>[2x]EEDELYRQSLEIISRYLREQATGAKDTKPMGRSGATSRKALETLRRVGDGVQRNHET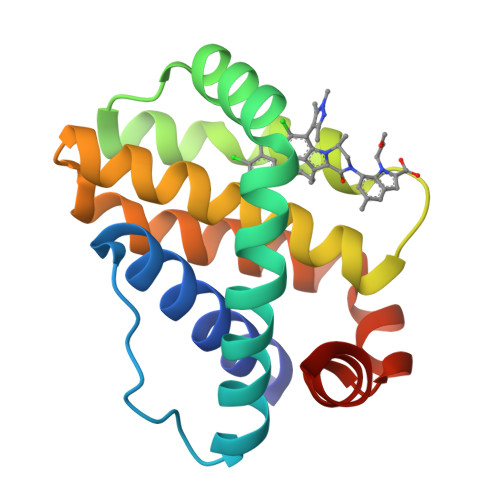AFQGMLRKLDIKNEDDVKSLSRVMIHVFSDGVTNWGRIVTLISFGAFVAKHLKTINQESCIEPLAESITDVLVRTKRDWLVKQRGWDGFVEFFHV>[2x]MSKDKVTVITSPSTEELVSLVNSALLEEAMLTIFARCKVHYDGRAKSELGSGDRVIIVKPDGSFLIHQSKKREPVNWQPPGSRVRLELRENPVLVSIRRKPRETLEVELEEVYMVSVFRAEDYEELALTGSEAEMAELIFENPEVIEPGFKPLFREKAIGTGIVAV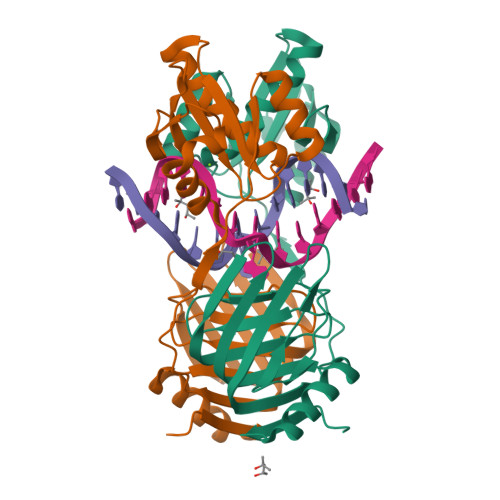LGRDSDGNIVVLELKRRRAELHAVRQLKSYVEILREEYGDKVRGILVAPSLTSGAKRLLEKEGLEFRKLEPPKRDSKKKGRQKTLF>[3x]MADGFFKQLTLPSGQVVTVSEGRGE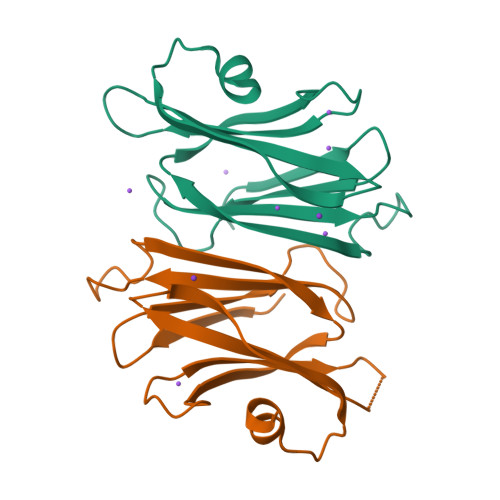PASTGSYDVRLYSGANPQFPLDQFIDGKVLPRDGSIKELKLLDLNGDKQPELIVVVESAGSGSYLSADAFTLNPQEGLDSFNHVEGLAPNEDVIQALKTPRDLEHHHHHH(2~{R})-2-phenylpiperidine-1-carbaldehyde | C12 H15 N O | 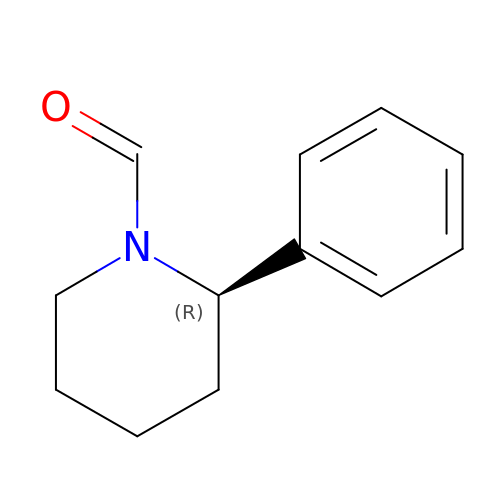MUZIXORETQNNBG-GFCCVEGCSA-N> SYYIDADLLREIKQHLKQ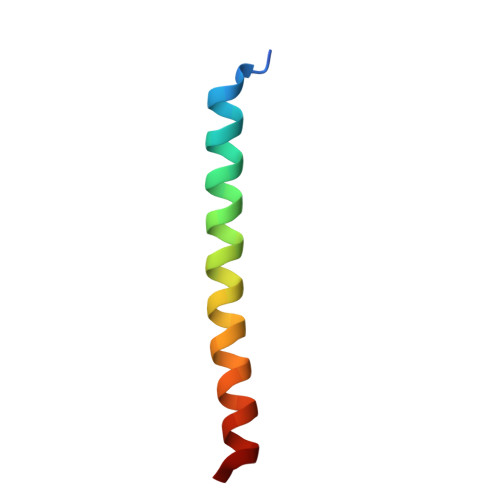QQEGLSHLISIIKDDLEDIKLV>[4x]VKLAGNSSLCPVSGWAPLSKDNSVRIGSKGDVFVIREPFISCSPLECRQFFLTQGALLNDKHSNGTIKDRSPYRTLMSVPIGSVPSPYNARFESIAWSASACHDGINWLTIGITGPDSGAVAILKYNGIITDTIKSWRNNILRTQESECACVNGSCFTIMTDGPSDGQASYKIFRIEKGKIIKSVEMKAPNYHYEECSCYPDSSEITCVCRDNWHGSNRPWV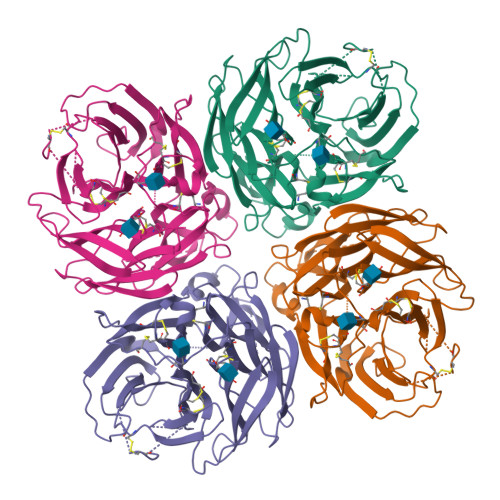SFNQNLEYQMGYICSGVFGDNPRPNDKTGSCGPVSSNGANGVKGFSFKYGNGVWIGRTKSISSRKGFEMIWDPNGWTGTDNKFSIKQDIVGINEWSGYSGSFVMHPELTGLDCIVPCFWVELIRGRPEENTIWTSGSSISFCGVNSDTVGWSWPDGAELPFTIDK> LDTSWKEATLPQVKAMLQKDTGKVSGDTVTYSGKTVHVVAAAVLPGFPFPSFEVHDKKNPTLDIPAGATVDVTFINTNKGFGHSFDITQKTPPFAVMPVIDPIVAGTGFSPVPKDGKFG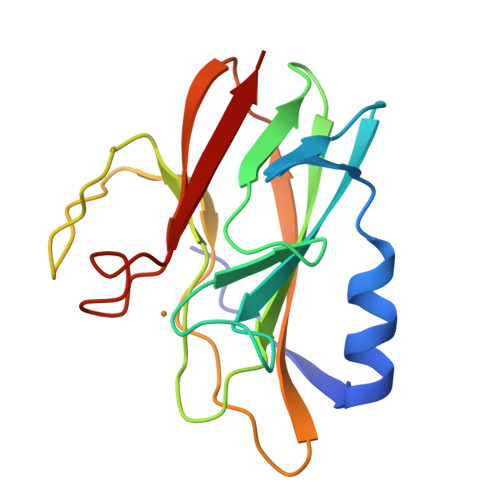YTNFTWHPTAGTYYYVCQIPGHAATGMFGKIVVK>QQASTLPDLAEQFAPPDVAPPLLIKLVEAIEKKGLECSTLYRTQSSSNPAELRQLLDCDTASLDLEMFDVHVLADAFKRYLLDLPNPVIPVAVSSELISLAPEVQSSEEYIQLLKKLIRSPSIPHQYWLTLQYLLKHFFKLSQTSSKNLLNARVLSELFSPLLFRFPAASSENTEHLIKIIEILISTKWNERQ[2x]

The N-terminal domains of p85α include an SH3 domain, capable of binding to proline-rich sequences, and a BH (breakpoint cluster region homology) domain. The BH domain can bind to and regulate several GTPases including Rab5, Rac1 and Cdc42. In addition, the p85α BH domain, either alone or together with the SH3 domain, can bind to and positively regulate PTEN activity. The p85α BH domain also exhibits Rab5 GAP activity to stimulate Rab5-mediated GTP hydrolysis required to inactivate Rab5-mediated protein trafficking functions.

To determine if the patient-derived p85α BH domain mutations impacted the overall folded structure of the BH domain, several of these BH domain mutants were crystalized and their structures were determined using X-ray crystallography. X-ray diffraction data collection and structure refinement statistics for bovine p85α (105–319) mutants (E137K, E217K, R262T, E297K) are provided in Supplementary Table S1. In contrast, several of the p85α mutants (E137K, K288Q, E297K) showed near wild type binding to PTEN, and either had enhanced (K288Q) or reduced (E297K, E137K) ability to stimulate PTEN lipid phosphatase activity. Three BH domain mutants, I177N, E217K and E297K, all showed significantly increased Rab5-GAP activity, whereas the E137K mutant had reduced activity. The location of cancer patient-derived p85α BH mutations with significant impacts on Rab5 binding (I177, E217) and/or regulation (E137, I177, E217, E297) are shown in the modeled p85α BH domain: Rab5 complex. These mutation sites are located in regions of the p85α BH domain, well away from the Rab5 binding pocket. Further, crystal structure determinations for several of these mutant BH domains indicated that no major structural alterations were present. No significant differences in protein flexibility were observed for any of the mutant proteins, suggesting that the mutations did not alter the rigidity of the domain.>[2x]ATDVIAQRKAILKQMGEATKPIAAMLKGEAKWDQAVVQKSLAAIADDSKKLPALFPADSKTGGDTAALPKIFEDK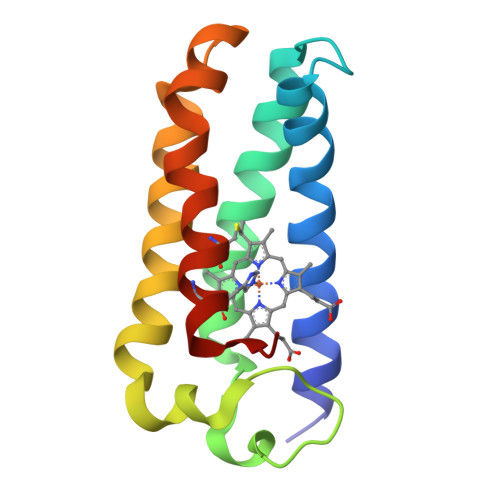AKFDDLFAKLAAAATAAQGTIKDEASLKANIGGVLGNCKSCHDDFRAKKS HMGR (3-hydroxy-3-methylglutaryl-coenzyme A reductase) is the rate limiting enzyme of the eukaryotic mevalonate pathway successfully targeted by statins to treat hypercholesterolemia in humans. As HMGR inhibitors have been shown to be herbicidal, HMGR could represent a mode of action target for the development of herbicides. Here, we present the crystal structure of a HMGR from Arabidopsis thaliana (AtHMG1) which exhibits a wider active site than previously determined structures from different species. By contrast, the conserved extracellular domain of AtHMG1 shares ~54% sequence identity with HsHMGCR and strictly conserved catalytic residues.

To develop plant-specific statins and mitigate off-target effects, we solved the crystal structure of the core domain of apo AtHMG1 and in complex with pitavastatin to resolutions of 1.9 and 2.1 Å, respectively, in space groupI 41 2 2. Conserved polar interactions occur with the residues local to the cis loop Arg296, Ser390, Asp396, Lys397, Lys398, Asn461 (HsHMGCR Arg590, Ser684, Asp690, Lys691, Lys692, Asn755) and a salt-bridge between the terminal carboxylate of the HMG moiety with Lys441 (HsHMGCR Lys735). The fluorophenyl group of pitavastatin maintains conserved stacking interactions with Arg296 (HsHMGCR Arg590) and hydrophobic interactions between the quinoline and cyclopropyl moiety with residues Leu268, Ile389, Leu558, Asp561 (HsHMGCR Leu562, Val683, Leu853, Asp856). This complex structure however also revealed two notable differences between the binding mode of class II statins in AtHMG1 and HsHMGCR; (i) loss of hydrogen bonding to the O5-hydroxyl group of the HMG moiety of statins from Glu265 (HsHMGCR Glu559), despite a slight shift of Glu265 towards the bound inhibitor, and (ii) the loss of hydrophobic interactions with Gly266, His458 and Ile562 (HsHMGCR Gly560, His752 and Leu857). Attempts were made to crystallise type I statins; however, electron density for these ligands was ambiguous. Modelling with AtHMG1 revealed more varied poses of the analogues, with similar affinities between the most favourable binding modes. These binding modes are possibly facilitated by a wider active site and flexibility in the Lβ2-Lα1 loop region and might account for the difficulty we had in obtaining co-crystal structures for AtHMG1. Our insights from the crystal structure of a model plant HMGR and the binding mode of pitavastatin provided the opportunity to rationally design plant-specific inhibitors.

> ENLYFQISRASGDAWDLADTIDDDDHRLVTCSPPTPIVSVAKLPNPEPIVTESLPEEDEEIVKSVIDGVIPSYSLESRLGDCKRAASIRREALQRVTGRSIEGLPLDGFDYESILGQCCEMPVGYIQIPVGIAGPLLLDGYEYSVPMATTEGCLVASTNRGCKAMFISGGATSTVLKDGMTRAPVVRFASARRASELKFFLENPENFDTLAVVFNRSSRFARLQSVKCTIAGKNAYVRFCCSTGDAMGMNMVSKGVQNVLEYLTDDFPDMDVIGISGNFCSDKKPAAVNWIEGRGKSVVCEAVIRGEIVNKVLKTSVAALVELNMLKNLAGSAVAGSLGGFNAHASNIVSAVFIATGQDPAQNVESSQCITMMEAINDGKDIHISVTMPSIEVGTVGGGTQLASQSACLNLLGVKGASTESPGMNARRLATIVAGAVLAGELSLMSAIAAGQLVRSHMKYNRSSRDISGATTTTTTTT> MSEKHPGPLVVEGKLTDAERMKHESNYLRGTIAEDLNDGLTGGFKGDNFLLIRFHGMYQQDDRDIRAERAEQKLEPRHAM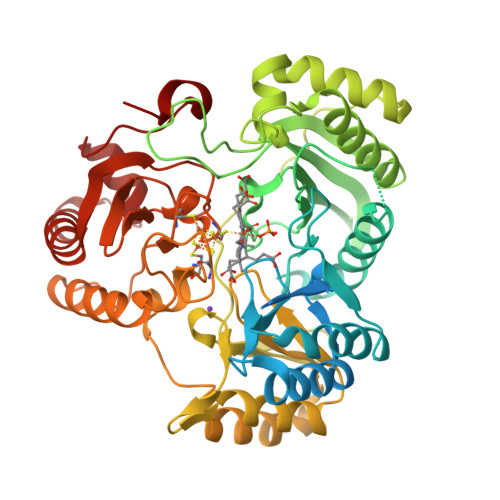LLRCRLPGGVITTKQWQAIDKFAGENTIYGSIRLTNRQTFQFHGILKKNVKPVHQMLHSVGLDALATANDMNSNVLCTSNPYESQLHAEAYEWAKKISEHLLPRTRAYAEIWLDQEKVATTDEEPILGQTYLPRKFKTTVVIPPQNDIDLHANDMNFVAIAENGKLVGFNLLVGGGLSIEHGNKKTYARTASEFGYLPLEHTLAVAEAVVTTQRDWGNRTDRKNAKTKYTLERVGVETFKAEVERRAGIKFEPIRPYEFTGRGDRIGWVKGIDDNWHLTLFIENGRILDYPARPLKTGLLEIAKIHKGDFRITANQNLIIAGVPESEKAKIEKIAKESGLMNAVTPQRENSMACVSFPTCPLAMAEAERFLPSFIDNIDNLMAKHGVSDEHIVMRVTGCPNGCGRAMLAEVGLVGKAPGRYNLHLGGNRIGTRIPRMYKENITEPEILASLDELIGRWAKEREAGEGFGDFTVRAGIIRPVLDPARDLWD>MGRKKIQIQRITDERNRQVTFTKRKFGLMKKAYELSVLCDCEIALIIFNHSNKLFQYASTDMDKVLLKY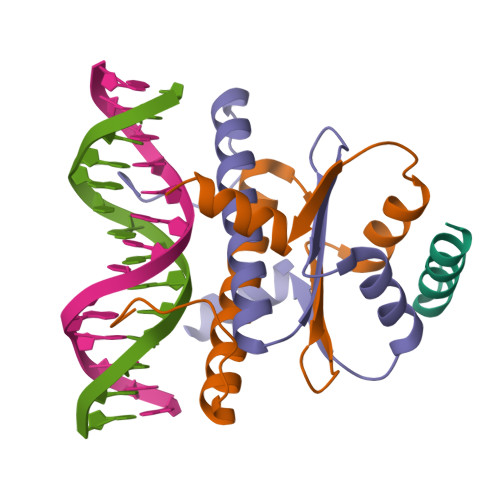TEYNEPHESRTNADIIETLRKKGFNG[4x];>[2x]WGSGEVKQKLQEFLLSKS>MEIDFEDDIDFDVYFRKTKAATILTKSTLENQNWRATTLPTDFNYNVDTLVQLHLKP[2x];>[2x]MGSSHHHHHHSQDPMGAERRLLSIKEAFRLAQQPHQNQAKLVVALSRTYRTMDDKTVFHEEFIHYLKYVMVVYKREPAVERVIEFAAKFVTSFHQSDMEDDEEEEDGGLLNYLFTFLLKSHEANSNAVRFRVCLLINKLLGSMPENAQIDDDVFDKINKAMLIRLKDKIPNVRIQAVLALSRLQDPKDDECPVVNAYATLIENDSNPEVRRAVLSCIAPSAKTLPKIVGRTKDVKEAVRKLAYQVLAEKVHMRAMSIAQRVMLLQQGLNDRSDA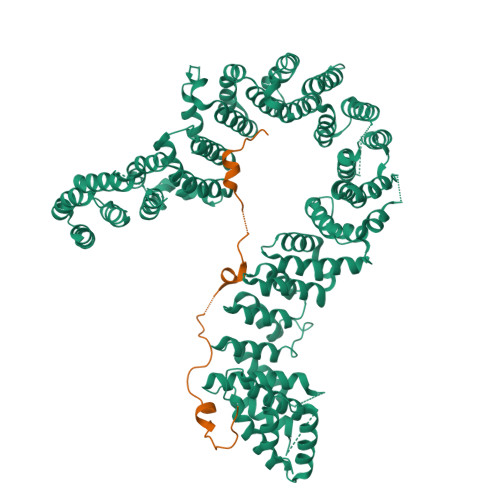VKQAMQKHLLQGWLRFSEGNILELLHRLDVENSSEVAVSVLNALFSITPLSELVGLCKNNDGRKLIPVETLTPEIALYWCALCEYLKSKGDEGEEFLEQILPEPVVYADYLLSYIQSIPVVNEEHRGDFSYIGNLMTKEFIGQQLILIIKSLDTSEEGGRKKLLAVLQEILILPTIPISLVSFLVERLLHIIIDDNKRTQIVTEIISEIRAPIVTVGVAETLQKCLILCYELLKQMSISTGLSATMNGIIESLILPGIISIHPVVRNLAVLCLGCCGLQNQDFARKHFVLLLQVLQIDDVTIKISALKAIFDQLMTFGIEPFKTKKIKTLHCEGTEINSDDEQESKEVEETATAKNVLKLLSDFLDSEVSELRTGAAEGLAKLMFSGLLVSSRILSRLILLWYNPVTEEDVQLRHCLGVFFPVFAYASRTNQECFEEAFLPTLQTLANAPASSPLAEIDITNVAELLVDLTRPSGLNPQAKTSQDYQALTVHDNLAMKICNEILTSPCSPEIRVYTKALSSLELSSHLAKDLLVLLNEILEQVKDRTCLRALEKIKIQLEKGNKE> MKMKRQEYVNTYGPTTGDKVRLGDTDLWAEVEHDYTVYGEELKFGAGKTIREGMGQSNSPDENTLDLVITNALIIDYTGIYKADIGIKNGKIHGIGKAGNKDMQDGVTPHMVVGVGTEALAGEGMIITAGGIDSHTHFLSPQQFPTALANGVTTMFGGGTGPVDGTNATTITPGVWNLHRMLRAAEEYGMNVGLLGKGNSSSRAQLVEQVKAGAIGFKLHEDWGTTPSAIDHCLSVADEYDVQVCIHTDTVNEAGYVDDTLRAMNGRAIHAYHIEGAGGGHSPDVITMAGEVNILPSSTTPTIPY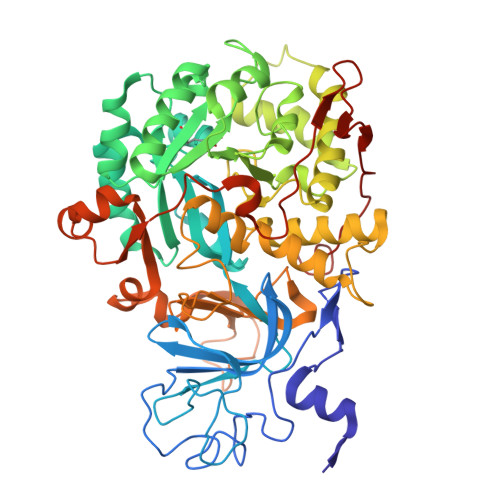TINTVAEHLDMLMTCHHLDKRIREDLQFSQSRIRPGSIAAEDTLHDMGVIAMTSSDSQAMGRAGEVIPRTWQTADKNKKEFGRLTEEKGDNDNFRIKRYISKYTINPAITHGVSEYIGSVEEGKIADLVVWNPAFFGVKPKIIIKGGMVVFSEMGDSNASVPTPQPVYYREMFGHHGKAKFDTSITFVSKVAYENGIKEKLGLERKVLPVKNCRNVTKKDFKFNNTTAKITVNPETFEVFVNGKLCTSKPATEVALASRYTFF>[8x]MRTPDIFIKATGRFLPETVSVEWAVEQGHYSAEDAELHELGGAAVAGDTPAPDMALWAAQQAVKRCGHRPEDLGLLLYVDSWHQGPDGWQPQYYLQRHLVGGDVLAVEIQQGCNGMFSALELAAAHLRAGPRPGSALVVAADNFGTPLFDRWTTGPGYIAGDGAGAVVLTTEPGFARLLAVRSLAVPEAEQMHRGAEPLFPPGATIGRPLNFTSRNAAFRELSLTEGLGTGALMRVHQRTLEVVEKTLSEAGITLGDITRVAYMNFSREIVEQRCMAALGLPMSASTWEFGRKLGHLGASDQVVALDELVTTGELGPGDHLLMLGMGPGVTLSCAVVKVLTPAPWSD

Chlorothricin (CHL) belongs to a spirotetronate antibiotic family produced by Streptomyces antibioticus that inhibits pyruvate carboxylase and malate dehydrogenase. A previous study reported that ChlB3 is involved in the conversion of 6-methylsalicyl-S-ChlB1-ACP to 6-methylsalicyl-S-ChlB2 with catalytic efficiency kcat/Km = 1690.70 mM−1 min−1. ChlB3 is a dimer having the same active sites as CerJ (a structural homologous enzyme) and uses a KSIII-like fold to work as an acyltransferase. Structural comparison indicated that ChlB3 belongs to FabH family and showed 0.6–2.5 Å root mean square deviation (RMSD) with structural homologous enzymes.

In the current study, the crystal structure of ChlB3 was solved at 3.1 Å-resolution and a catalytic mechanism was proposed on the basis of conserved residues of structurally related enzymes. The protein structure was present in the space group of P212121 with four dimers per asymmetric unit. The refined model of ChlB3 contained 334 residues in each monomer and no electron density was observed for its 197–201 and 227–230 residues. ChlB3 structure is organized as a homodimer and each monomer having its own active site. Each ChlB3 monomer has a seven-layered core composed of two layers of helices interspersed by five layers of sheet, with several connecting loop regions around the core. The core region features an internal duplication of two segments (14–183 and 184–339) that are comparable in structure except at their loop regions, although there is no major sequence similarity between the two halves. A total of 2627.6 Å area is buried in the dimer interface of ChlB3 protein. The main chains of Thr205, Arg215, Gly112, Ala185, Arg239, Gln110, Gln92, Gln90, Gly102, Asp103, Trp89, Gly85 and Glu190 are involved in hydrogen bonding at the monomer-monomer interface. Generally, in KSIII enzymes cystine is responsible for the transacylation process, although histidine and aspartic acid catalytic residues crucial for Claisen-like condensation. ChlB3 catalytic triad (Cys113, His296 and Asp301) as shown in Figure 2C, significantly differs in electrostatic character and geometry, despite the catalytic cysteine (Cys113) occupying the same position as those seen in both structurally related enzymes. The volume of active site cavity, as calculated by the program CASTp 3.0, was 934 Å3.>HMAQETIVIGLAADSGCGKSTFMRRLTSVFGGAAKPPKGGNPDSNTLISDTTTVICLDDYHSLDRYGRKEQKVTALDPRANDFDLMYEQVKALKNGIAVEKPIYNHVTGLLDPPELIQPPKILVIEGLHPMFDERVRDLLDFSIYLDISNEVKFAWKIQRDMAERGHSLESIKASIEARKPDFDAFIDPQKQYADAVIEVLPTTLIPDDNEGKVLRVRLIMKEG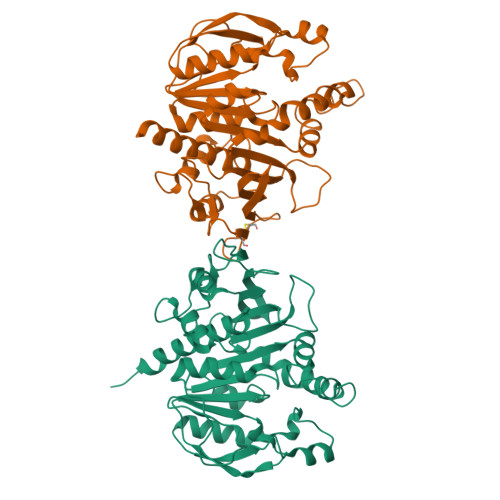VKYFSPVYLFDEGSTISWIPCGRKLTCSYPGIKFNYEPDSYFDHEVSVLEMDGQFDRLDELIYVESHLSNLSTKFYGEVTQQMLKHADFPGSNNGTGLFQTIVGLKIRDLYEQLIANKATARAEAKA[2x]>MATDWTDNRKNLMLFAGRAHPELADQVAKELDVAVTAQTARDFANGEIFVRFDESVRGCDAFVLQSHPAPLNQWLMEQLIMIDALKRGSAKRITAILPFYPYARQDKKHRGREPISARLVADLLKTAGADRIVSVDLHTDQIQGFFDGPVDHMRAQKLLTGYIGEHYADEDMVVVSPDSGRVRVAEKWADSLGGVPLAFIHKTRDPLVPNQVKSNRVVGDVKGKTCILTDDMIDTGGTIAGAVNLLREDGAKDVIIAATHGVLSDPAPQRLAECGAREVIVTNTLPITEDKRFPQLTVLSIAPLLANTIRAVFENGSVTGLFDGSA[3x]

In this context, phosphoribosylpyrophosphate (PRPP) is an essential molecule for the biosynthesis of purine and pyrimidine nucleotides, of NAD(P), as well as of the amino acids histidine and tryptophan. The M. tuberculosis PrsA (MtPrsA) catalyzes the Mg2+-dependent conversion of ribose 5-phosphate (R5P) to PRPP using ATP, and is the solely enzyme responsible for PRPP synthesis in MTB. In this context, we report the structural and biochemical characterization of the PrsA enzyme from M. smegmatis (MsPrsA; 87% identity with MtPrsA), that is the first X-ray crystal structure of a mycobacterial PrsA ever determined. Our results demonstrate that the enzyme is a Class I PRPP synthetase and shows the typical structural architecture common to other PrsAs.

The final MsPrsA structure contains residues from Arg9 to Gly316, with no electron density observed for the first eight amino-acids and for the stretch Arg204-Lys213. A Matthews parameter and a solvent fraction of 2.11 Å Da-1 and 41.76%, respectively, were calculated indicating the presence of three protein subunits in the asymmetric unit. The physiological hexamer was generated by applying a two-fold crystallographic symmetry operators to the trimer. The resulting hexamer is endowed with a 32-point symmetry with a two-fold axis perpendicular to a three-fold axis and shows the subunits arranged in a propeller-shaped cyclic assembly with the N-terminal domains oriented toward the inner side of the hexamer, close to the three-fold axis. Each domain consists of an ɑ/β fold built on a central five-stranded parallel β-sheet surrounded by four ɑ-helices with the N-terminal domain (residues Thr139-Phe146) containing an additional 310 helix. In all the subunits of MsPrsA one molecule of acetate (ACT) sits in the phosphate binding pocket of the ribose-5-phosphate binding site and makes specific contacts with residues defining the R5P binding loop (amino-acids Asp230-Thr238). As the crystal structure we determined is the one of the ligand-free form, we analysed the R5P and ATP binding mode by modelling the ligands in their respective binding sites by optimal structural superposition and energy minimization. While the R5P binding site does not reveal any significant peculiarity in MsPrsA and is confirmed as highly structurally conserved, significant differences are observed in the case of the ATP binding compared to the human ortholog. More significant instead are the two differences observed in the ATP binding pocket where the recognition of the ribose portion of the nucleotide is completed in the mycobacterial enzyme with a Glutamic residue that replaces an Alanine in the equivalent position in the human enzyme (Glu113 vs Ala105).{(1R,2R)-3-oxo-2-[(2Z)-pent-2-en-1-yl]cyclopentyl}acetic acid | C12 H18 O3 | 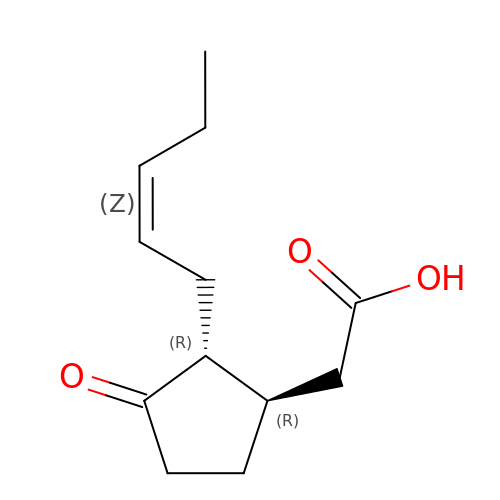ZNJFBWYDHIGLCU-HWKXXFMVSA-N> SHHHHHHHHHHSKQKNEESKKRQWALEDFEIGRPLGKGKFGNVYLAREKQSKFILALKVLFKAQLEKAGVEHQLRREVEIQSHLRHPNILRLYGYFHDATRVYLILEYAPLGTVYRELQKLSKFDEQRTATYITELANALSYCHSK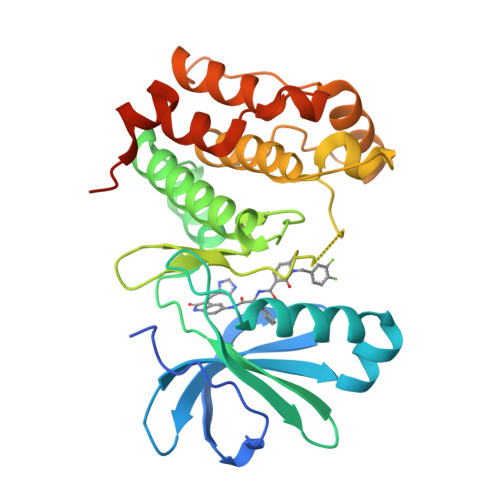RVIHRDIKPENLLLGSAGELKIADFGWSVHAPSSRRTTLCGTLDYLPPEMIEGRMHDEKVDLWSLGVLCYEFLVGKPPFEANTYQETYKRISRVEFTFPDFVTEGARDLISRLLKHNPSQRPMLREVLEHPWITANSSKPSNCQNKESASKQS>[2x]GPGEKLELRLKSPVGAEPAVYPWPLPVYDKHHDAAHEIIETIRWVCEEIPDLKLAMENYVLIDYDTKSFESMQRLCDKYNRAIDSIHQLWKGTTQPMKLNTRPSTGLLRHILQQVYNH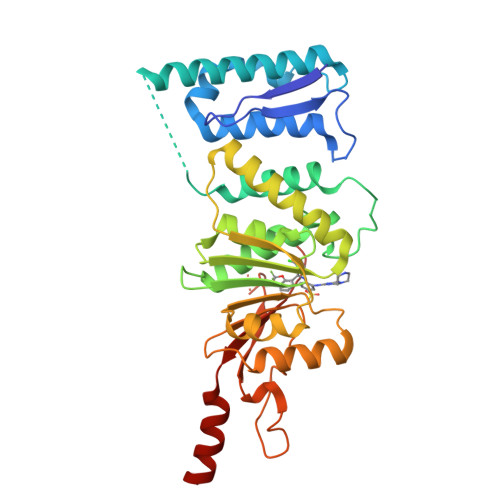SVTDPEKLNNYEPFSPEVYGETSFDLVAQMIDEIKMTDDDLFVDLGSGVGQVVLQVAAATNCKHHYGVEKADIPAKYAETMDREFRKWMKWYGKKHAEYTLERGDFLSEEWRERIANTSVIFVNNFAFGPEVDHQLKERFANMKEGGRIVSSKPFAPLNFRINSRNLSDIGTIMRVVELSPLKGSVSWTGKPVSYYLHTIDRTILENYFSSLKNPG> MLPQRLHPSRLLALALFSLVLGLAGCQTKPPQTGLSAEQIAVLQEQGFELRDEGWPGSMSSKVLFGNNLDRLNPDSRNTLTKIARALLAVDIDKV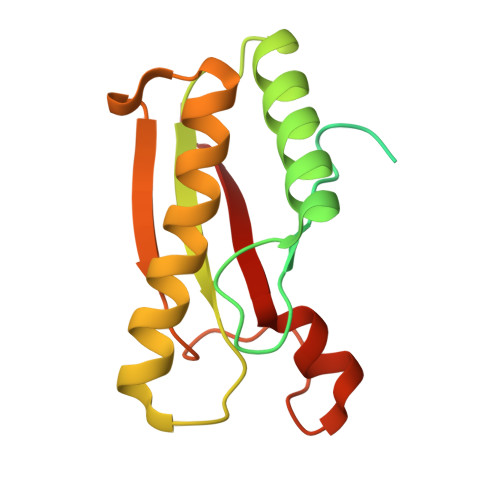RLEGHTDNYGDEGYNQKLSERRAESVAAVFREAGMPAANIEVRGLGMSKPVADNKTRAGRSENRRVAIIVPAE>MFNYESILINEDVVSEMTIEDAKKLKPYWNVQIANFKKSSKEPMFTLLQMAILLNKKDIVGYLLARRGLDINALSRNNQTALMIACDKKV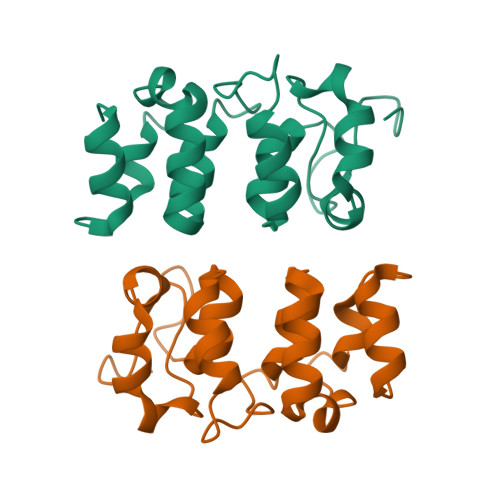PLDWIEAILKRGGDLGINIKDDYEQTALDKCNFNSKAYHLLLKYGA[2x]> MGTQQKDVTIKSDAPDTLLLEKHADYIASYGSKKDDYEYCMSEYLRMSGVYWGLTVMDLMGQLHRMNKEEILVFIKSC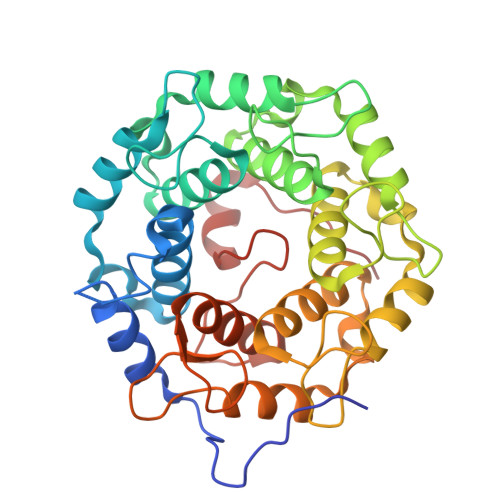QHECGGVSASIGHDPHLLYTLSAVQILTLYDSIHVINVDKVVAYVQSLQKEDGSFAGDIWGEIDTRFSFCAVATLALLGKLDAINVEKAIEFVLSCMNFDGGFGCRPGSESHAGQIYCCTGFLAITSQLHQVNSDLLGWWLCERQLPSGGLNGRPEKLPDVCYSWWVLASLKIIGRLHWIDREKLRSFILACQDEETGGFADRPGDMVDPFHTLFGIAGLSLLGEEQIKPVSPVFCMPEEVLQRVNVQPELVS>MRYNQGCQLTAFFIGGNMKIVKHDGYNDIFNGGADGSPKPFFMSDASYHVGSFYNDNATAKRIVDVIPEEMVTAGFKISGVKDEKEFKSLWDSYKIDPSLVDALCWARLYGGAAIVAIINDNRMLTSPVKPGAKLEGVRVYDRFAITIEKRVTNARSPRYGEPEIYKVSPGDNIQPYLIHHTRIFIADGERVTPQMRKQNQGWGASVLNKSLIDAICDYDYCESLATQILRRKQQAVWKVKGLAEMCDDDDAQYAARLRLAQVDDNSGVGRAIGIDAETEEYDVLNSDISGVPEFLSSKMDRIVSLSGIHEIIIKNKNVGGVSASQNTALETFYKLVDRKREEDYRPLLEFLLPFIVDEQEWSIEFEPLSVPSKKEESEITKNNVESVTKAITEQIIDLEEARDTLRSIAPEFKLKDGNNINIREPEEPTEPEPGLGEKLEDEN[2x];>[2x]MGVIMNQETLIAAVEQMRKLVPALRKVPDETLYAWVEMAELFVCQKTFKDAYVKAIALYALHLAFLDGALKGEDEDLESYSRRVTSFSLSGEFSQTFGEVTKNQSGNMMLSTPWGKMFEQLKARRRGRFALMTGLRGGCH;> MNYSQIERMARKGVAFFTDPSRPMNLIKQGEYGYDENGFEIPPMEQVIPISGATRRPNAREIDGETIRASDILGIFNNDHEINEGDYIEIDGIRHVVVDARPVQASLEPVAYRPVLRRVSVGG;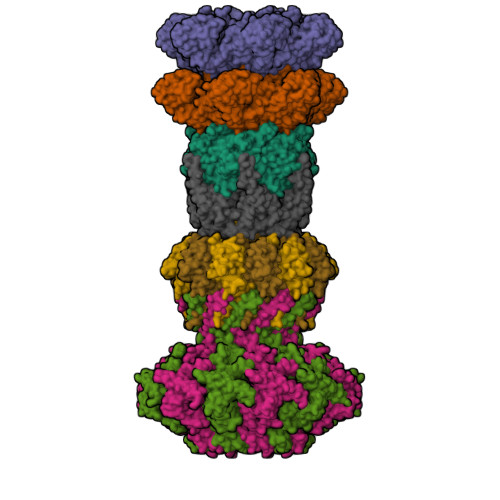> MHYELSAAARAAFLSKYRDFPHYMENRNFTPPKDGGMWLRFNYIEGDTLYLSIDRKCKSYIAIVQIGVVFPPGSGVDEARLKAKEIADFFKDGKMLNVGYIFEGAIVHQIVKHESGWMIPVRFTVRVDTKET;>[2x]MHLPNGAQIFVETSRGEEIEATAVTNEKNPVATVASKGDLAKGDYVIVTQSTWAKMVSRVLIVTDAQETSITLAGIDTSDTLVFPAGGTMSFAKITGWTEIPCVQEIGQDGGEQQYYTYQCLSDDKEQQIPTFKSAISLTYTFAHEFDNPIYQILRKLDSSGQVTAVRMYVPKASEMRMWAGILSFNDIPSTQVNEMETVELAVSLKGDFTFISSTLASPGA> 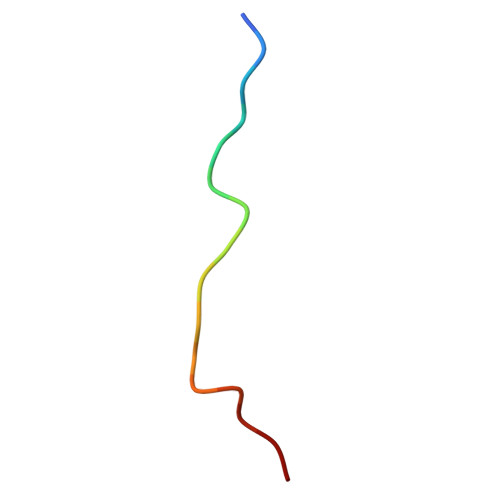MLARRKPVLPALTINP>[4x]MNLKDKILGVAKELFIKNGYNATTTGEIVKLSESSKGNLYYHFKTKENLFLEILNIEESKWQEQWKKEQIKAKTNREKFYLYNELS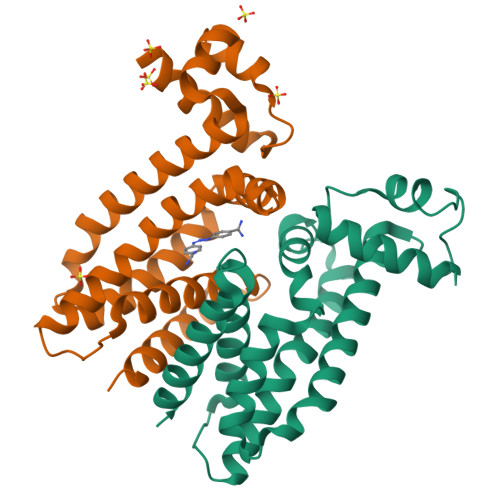LTTEYYYPLQNAIIEFYTEYYKTNSINEKMNKLENKYIDAYHVIFKEGNLNGEWSINDVNAVSKIAANAVNGIVTFTHEQNINERIKLMNKFSQIFLNGLSKHHHHHH2-methyl-1-nitro-3-[(tetrahydro-3-furanyl) methyl] guanidine | C7 H14 N4 O3 | 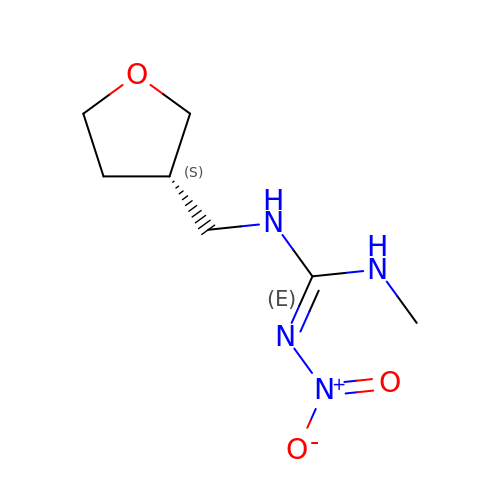YKBZOVFACRVRJN-LURJTMIESA-N> AAHHSSGHMEATLGSGNLRQAVMLPEGEDL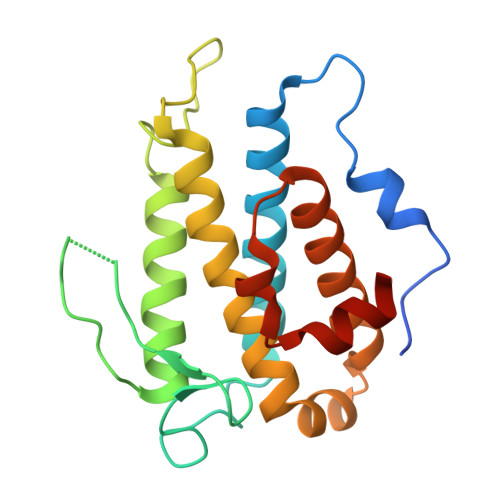NEWIAVNTVDFFNQINMLYGTITEFCTEASCPVMSAGPRYEYHWADGTNIKKPIKCSAPKYIDYLMTWVQDQLDDETLFPSKIGVPFPKNFMSVAKTILKRLFRVYAHIYHQHFDSVMQLQEEAHLNTSFKHFIFFVQEFNLIDRRELAPLQELIEKLGSKDR>ATLPAGASQVPTTPAGRPMPYAIRPMPEDRRFGYAIVGLGKYALNQILPGFAGCQHSRIEALVSGNAEKAKIVAAEYGVDPRKIYDYSNFDKIAKDPKIDAVYIILPNSLHAEFAIRAFKAGKHVMCEKPMATSVADCQRMIDAAKAANKKLMIGYRCHYDPMNRAAVKLIRENQLGKLGMVTTDNSDVMDQNDPAQQWRLRRELAGGGSLMDIGIYGLNGTRYLLGEEPIEVRAYTYSDPNDERFVEVEDRIIWQMRFRSGALSHGASSYSTTTTSRFSVQGDKAVLLMDPATGYYQNLISVQTPGHANQSMMPQFIMPANNQFSAQLDHLAEAVINNKPVRSPGEEGMQDVRLIQAIYEAARTGRPVNTDWGYVR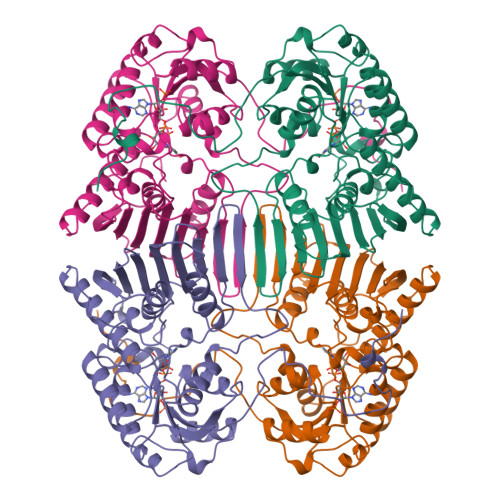QGGY[6x]> MALLAEHLLKPLPADKQIETGPFLEAVSHLPPFFDCLGSPVFTPIKADISGNITKIKAVYDTNPAKFRTLQNILEVEKEMYGAEWPKVGATLALMWLKRGLRFIQVFLQSICDGERDENHPNLIRVNATKAYEMALKKYHGWIVQKIFQAALYAAPYKSDFLKALSKGQNVTEEECLEKIRLFLVNYTATIDVIYEMYTQMNAELNYKV

Human glycolipid transfer protein (hsGLTP) forms the prototypical GLTP fold and is characterized by a broad transfer selectivity for glycosphingolipids (GSLs). In human GLTP, a glycolipid headgroup recognition centre located on the protein surface enables selective binding of the GSL head and ceramide amide groups via multiple specific interactions. Encapsulation of lipid chains within the hydrophobic pocket involves a cleft-like gating mechanism that results in two glycolipid-binding modes. To elucidate the structural dynamics of the GLTP–GSL dimer and associated adaptations, we comparatively analyzed nine novel crystal structures of wild-type GLTP (wtGLTP) and the sulfatide-specific mutants D48V and A47D/D48V complexed with N-lauroyl-containing monosulfatide (N-lauroyl-3-O-sulfo-galactosylceramide; hereafter referred to as 12:0 monoSF) and disulfatide (N-lauroyl-3,6-di-O-sulfo-galactosylceramide; hereafter referred to as 12:0 diSF) in different crystal forms and compared them with previously studied GLTP–24:1 monoSF complexes.

Disulfatide and all amino-acid residues of the GLTP recognition centre are clearly visible in the electron-density map. The protein structure displays no disturbance compared with wtGLTP complexed with monosulfatides. Hence, we can assume that the disulfatide found in the malaria parasite Plasmodium falciparum can also be bound by human GLTP. The first noticeable deviations in the surface contact areas occur in wtGLTP–disulfatide complexes, which probably indicate a slightly different mutual orientation of monomers compared with wtGLTP–monosulfatide complexes. Indeed, careful comparison reveals some monomer–monomer′ contact redistribution in the dimer in the region of the α6–α6′ and α2–α2′ protein interactions and lipid–protein′ contacts. To elucidate the dynamics of intermolecular interactions in the GLTP–disulfatide complex, we comparatively analyzed two crystal forms of wtGLTP and two crystal forms of the D48V mutant complexed with 12:0 diSF. The crystals of the wtGLTP–disulfatide complex represent ‘open’ and ‘closed’ conformations of the dimeric arrangement. Interestingly, ligand adaptations also emerge with wtGLTP complexes bound with disulfatide. In contrast, the 6-O-sulfo group adopts different conformations/positions that depend on the protein (wild type or D48V) or the crystal type.> MASPAVRKAISDAALQYAKPEGKIFQYGTAGFRMKADLLNTVVYAVGLLATLRSKKLSGQWIGVMVTAAHNPAEDNGVKLVDPMGEMLEAEWEAYATKLANAPLENIGDVYDELVKEIDVSMENPARVVFARDTRASGSRLIGVLSAALTATEAEFIDMKFMTTPQLHYVVRCKNTLGTQYEYGEPTEQGYYEKLAAAFKRVMRGVKVKGSLTVDCANGVGGPKLRELIKYLPEDTGLDIKIVNDDVINPDSLNFECGADYVKTKQRAPPSSKASILDRCASLDGDADRILYYFLDEGNVFRLLDGDRIATLAASFIGDLARSAGIAQKLKIGVVQTAYANGSSTEYIEKVLKLPSVCTNTGVKHLHHAAMRFDVGVYFEANGHGTITFSENALKTIKNTEPQSPAQQRSLECLQALTDLINQAVGDAISDMLLVEAILAHKGWTPKEWLATYTDLPSRLVRVEVAERSIFKAYDAERKLESPPGLQAKIDSLQSRYNKGRSFARASGTEDAVRVYAEAASRSEADDLATRVANAVRDAGTVKEILQAS

N-acetylphosphoglucosamine mutase (AGM1) catalyzes the interconversion of N-acetylglucosamine-6-phosphate (GlcNAc-6P) to N-acetylglucosamine-1-phosphate (GlcNAc-1P) in eukaryotes. This enzyme is a member of the α-d-phosphohexomutase superfamily of enzymes that catalyze intramolecular phosphoryl transfer on a range of phosphosugar substrates. The reaction catalyzed by AGM1 is the third step in the biosynthesis of UDP-GlcNAc from fructose-6-phosphate in the hexosamine pathway. Previously, AGM1 was shown to be an essential gene in the human fungal pathogen Aspergillus fumigatus and has been proposed as a drug target.

As expected, steady-state kinetics reveal that mutating Ser69 to alanine completely abolishes enzyme activity. Once it was clarified that Ser69 was the only residue being phosphorylated during catalysis, we exploited this catalytically impaired mutant to trap the bisphosphorylated intermediate that has been proposed for this class of phosphomutase. The protein was crystallized with Glc-1,6-bisP and the structure was refined to 1.9 Å resolution with a single protein molecule in the asymmetric unit. The overall structure of AfAGM1_S69A–Glc-1,6-bisP complex shows a closed conformation, compared with the open/semi-open conformations exhibited by the two monomers in the AfAGM1–GlcNAc-6P–Mg+2 complex. However, the inactive AfAGM1_S69A mutant–Glc-1,6-bisphosphate complex has an overall structure with a closed active site and represents the reaction intermediate with Glc-1,6-bisphosphate buried in the active pocket. The complete closure of the active site is achieved by the establishment of extensive hydrogen bond interactions between the reaction intermediate Glc-1,6-bisphosphate and the protein. In addition, the 1-phosphate group establishes hydrogen bond interactions with R33, H70, R289 and a water molecule, the 6-phosphate group makes hydrogen bond interactions with T29, R505, S507, T509, R514 and the backbone of G508, and the 3-OH and 4-OH groups of the sugar make hydrogen bond interactions with E380 and the backbone of V363. Thus, extensive hydrogen bond interactions are established with residues from all the domains resulting in a closed conformation. This provides a snapshot of the reaction either immediately after phosphoryl transfer to form the intermediate or before the second phosphoryl transfer to re-phosphorylate the enzyme. Although the inactive AfAGM1_S69A mutant–Glc-1,6-bisphosphate complex was crystallized in the presence of 10 mM MgCl2, the structure reveals the absence of this metal and the presence of a water molecule instead.> MSYKQTTYYPSRGNLVRNDSSPYTNTISSETNNSSTSVLSLQGASNVSLGTTGNQLYMGDLDPTWDKNTVRQIWASLGEANINVRMMWNNTLNNGSRSSMGPKNNQGYCFVDFPSSTHAANALLKNGMLIPNFPNKKLKLNWATSSYSNSNNSLNNVKSGNNCSIFVGDLAPNVTESQLFELFINRYASTSHAKIVHDQVTGMSKGYGFVKFTNSDEQQLALSEMQGVFLNGRAIKVGPTSGQQQHVSGNNDYNRSSS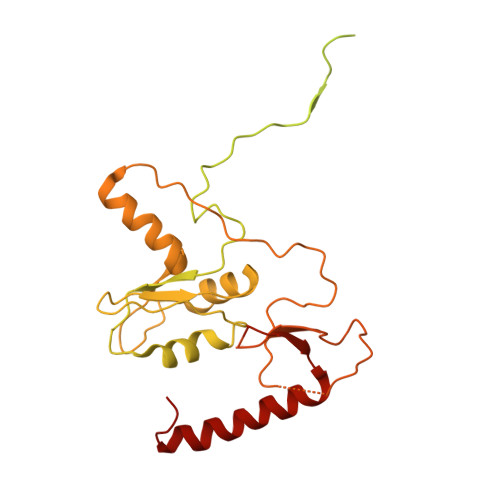SLNNENVDSRFLSKGQSFLSNGNNNMGFKRNHMSQFIYPVQQQPSLNHFTDPNNTTVFIGGLSSLVTEDELRAYFQPFGTIVYVKIPVGKCCGFVQYVDRLSAEAAIAGMQGFPIANSRVRLSWGRSAKQTALLQQAMLSNSLQVQQQQPGLQQPNYGYIPSSTCEAPVLPDNNVSSTMLPGCQILNYSNPYANANGLGSNNFSFYSNNNATNTQATSLLADTSSMDLSGTGGQQVIMQGSEAVVNSTNAMLNRLEQGSNGFMFA>[4x]MEEPEEPADSGQSLVPVYIYSPEYVSMCDSLAKIPKRASMVHSLIEAYALHKQMRIVKPKVASMEEMATFHTDAYLQHLQKVSQEGDDDHPDSIEYGLGYDCPATEGIFDYAAAIGGATITAAQCLIDGMCKVAINWSGGWHHAKKDEASGFCYLNDAVLGILRLRRKFERILYVDLDLHHGDGVEDTFSFTSKVMTVSLHKFSPGFFPGTGDVSDVGLGKGRYYSVNVPIQDGIQDEKYYQ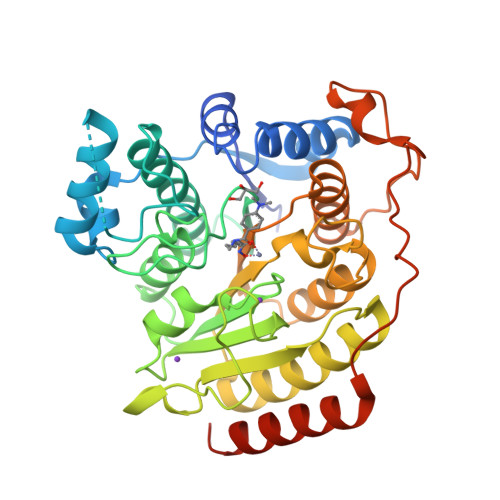ICESVLKEVYQAFNPKAVVLQLGADTIAGDPMCSFNMTPVGIGKCLKYILQWQLATLILGGGGYNLANTARCWTYLTGVILGKTLSSEIPDHEFFTAYGPDYVLEITPSCRPDRNEPHRIQQILNYIKGNLKHVVIEGRGSHHHHHH>MAGRITINGTSHEVNLSALPADISLNTFIREYAGLTGTKFMCQEGGCGVCVCTLTGIHPETGELRTWAVNSCLTLLNTCLGLEVTTSEGLGNKRVGYHAIQQRLAKMNGTQCGYCSPGIVMNMYGLLKSKGGKVTMEEVENSFGGNICRCTGYRPILDAMKSFAVDSNIQVPAECIDIEDLSTKKCPKTGQTCSGSCKKQQPKGSQLYPDGSRWSWPVSLGDLFAALQGAVKEKLPYMLVAGNTAHGVYRRSPDIKAFIDVSGLAELKGHKLSADNSSLTLGGNLSLSETMELCRQLENTKGFEYLSQVWQHLDWIANVPVRNAGTLAGNLSIKHAHPEFPSDVFIVLEALDAQVIVQEAVDKQQTVSLASYLGSSMEGKIIRGLVLRAYPKERFAFDSYKIMPRAQNAHAYVNAAFLVEFTADAKVKSARICFGGIHPEFVHATAIENLIRDKNPFENGLVEKAFGQLSTLLQPDAVLPDASPVYRRKLACGLFYKFLLKIAAQRKQGLGSRFVTGGSLLKRPVSSGQQSFETFQEHYPVTKATEKHEGLIQCSGEATYSNDLPTQHNQLWAAFVIAKKVGAKVTKVDTQPALDLPGVVAYLDAKDIPGPNYVGPKIRDQFFFPKDEELFATGEIKFYGQPVGIILANSNSLANRAAELVKLTYEGGAEEILPSLKAVLDKVGSEAGNNKRLEQPIKSTIDVLQLEEPFDVSSSGQLDMGLQYHYYMEPQTTVVLPFEGGLQVYAATQWMDLTQDTIANVLNLKSNDVQVKTRRIGGGYGGKATRCNLAAAAAALAAHKLNRPIRFVQSLESIMTSLGKRWAFHCDYDFFVQKSGKISGIVSRFYEDAGYLANESPIGHTVLLSKNCYEFSDNYKLDGYLVCTDSPSNTPCRAPGSVEGIAMMENIIEHIAFETGVDPADVRFANLLPAHKMGDMMPRFLESTKYRERKAEAIAHNKENRWHKRGLGLCIMEYQIGYFGQYPATVAIYHSDGTVVVSHGGIEMGQGMNTKISQVAAHTLGIPMEQVRIEASDTINGANSMVTGGAVGSETLCFAVRKACETLNERLKPVREEVKPENWQDLIQEAYNRKINLIASDQCKQGDMDPYSVCGLCLTEVELDVLTGNYIVGRVDILEDTGESLNPNVDIGQIEGAFMMGLGYWTSEQVIADPKTGECLTNRTWTYKPPGAKDIPTDLRIELLPKSPNKAGFMRSKATGEPAICLSI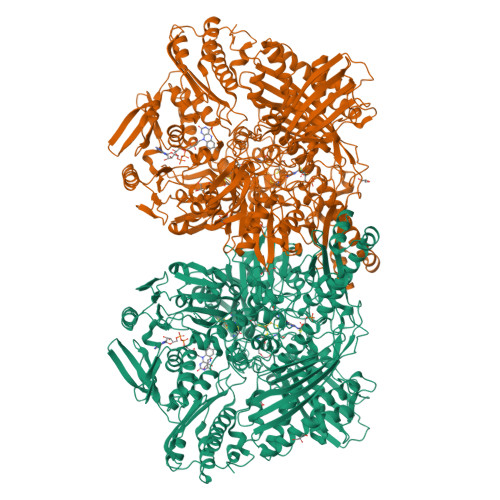AVAFALQQALQSARDDAGVPKSWVTLTAPMTPEHLVLHSGTEPSQFKLN[4x]> MDGGMWLMQQINGQVARMKSLGMQLEAADIYNPNGSSL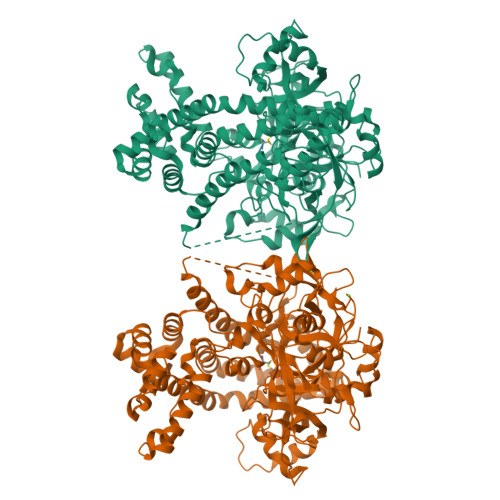KDAVVMFDGGCTGVLVSNQGLLLTNHHCGYDQIQKHSSVQHNYLKDGFWSYSLAEELVNPGLEVEIVDEITDVTAAVKKELERIKKPSGLEFLSPRYLSSLAPEIVGKKAASRPGYRYEIKAFYGGNRYYMFTKKVFRDVRLVAAPPSSIGKFGSDTDNWAWPRHTGDFSIFRLYADKNGNPAEYSKDNVPYRPKRWVKVNAQGVKEGDFALIMGYPGTTYKFFTADEVTEWSEIDNNIRIEMRGILQDVMLREMLADPKINIMYAAKYASSQNGYKRAQGANWAIRRRSLREIKLAQQQEVLAWAKQKGIATTEEAVRAISKAIEGRQDLRMRQRYLLEGILMGIEMSNAPAADSDIADHWDDPARREAGLQSIRKQFEAFFNKDYSPEVEKDQLAIALLTRYAERIPAEKQPISIREGIAEYGSAKAYVEMIFDKSIYASRERFEEFMKNPDRDRLLRDPMSRFAASVAYEHQKLAKEVAAFDAPLAAAQRSYVASVLDMKGQPNLAPDANLTLRFTYGEIKGYQPRDVVTYGAKSTLEGVMEKEDPNNWEYVVDPKLKALYEAKNYGRYANSDGSMPVNFCATTHTTGGNAGSPVMNARGELIGLNFDRNWEGVGGDIEYLPNYQRSIILDIRYLLFIIDKFAGCQRLIDEIQPQFHHHHHH> GGMAGQNPNMDQFEAYFKRADLDGDGRISGAEAVGFFQGSGLSKQVLAQIWSLSDRSHSGFLDRQNFYNSLRLVTVAQSKRDLTPEIVNAALNTPAAAKIPPP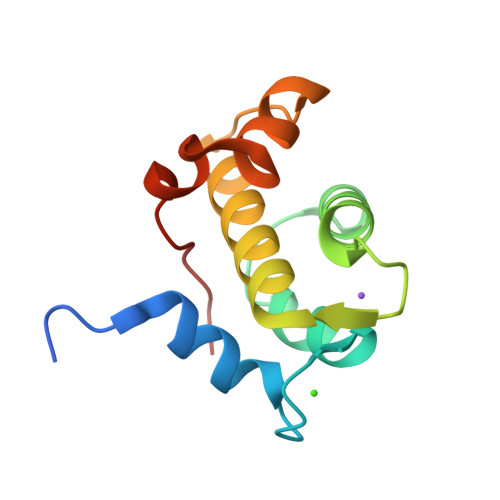KINLSA3-[C-[N'-(3-CARBAMIMIDOYL-BENZYLIDENIUM)-HYDRAZINO]-[[AMINOMETHYLIDENE]AMINIUM]-IMINOMETHYL]-BENZAMIDINIUM | 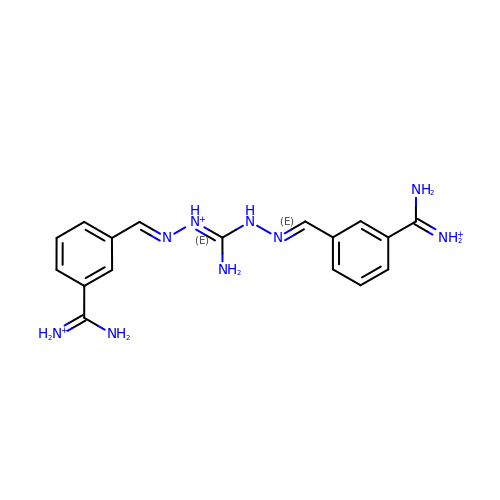C17 H22 N9 | NSHBIZYDZBQOQB-WDBPGAOMSA-Q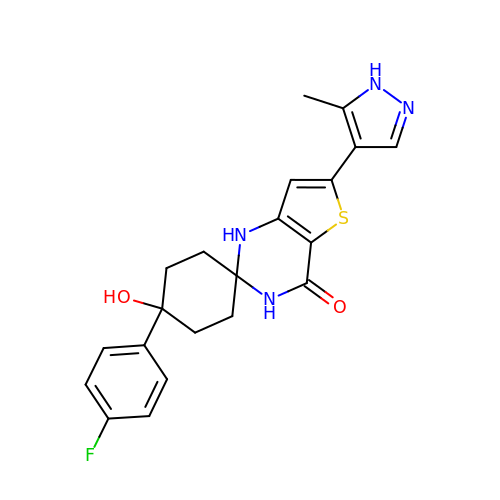(1s,4s)-4-(4-fluorophenyl)-4-hydroxy-6'-(5-methyl-1H-pyrazol-4-yl)-1'H-spiro[cyclohexane-1,2'-thieno[3,2-d]pyrimidin]-4'(3'H)-one | C21 H21 F N4 O2 S | NCRZDERILSVITP-OYRHEFFESA-N>QGPGGGGSVTCPGGQSTSNSQCCVWFDVLDDLQTNFYQGSKCESPVRKILRIVFHDAIGFSPALTAAGQFGGGGADGSIIAHSNIELAFPANGGLTDTVEALRAVGINHGVSFGDLIQFATAVGMSNCPGSPRLEFLTGRSSSSQPSPPSLIPGPGNTVTAILDRMGDAGFSPDEVVDLLAAHSLASQEGLNSAIFRSPLDSTPQVFDTQFYIE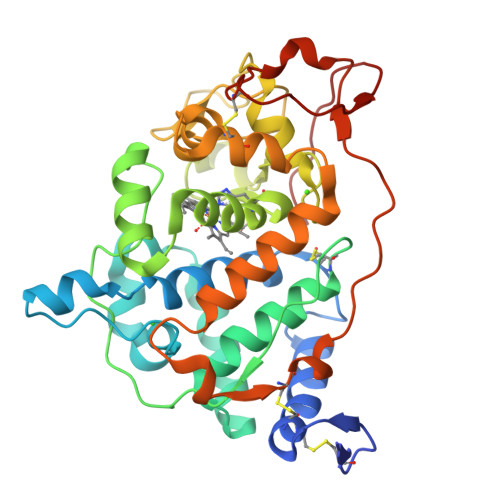TLLKGTTQPGPSLGFAEELSPFPGEFRMRSDALLARDSRTACRWQSMTSSNEVMGQRYRAAMAKMSVLGFDRNALTDCSDVIPSAVSNNAAPVIPGGLTVDDIEVSCPSEPFPEIAAASGPLPALAPAP[2x]>MAHHHHHHMTRAFNFSAGPATLPESVLRQAQAEMLDWHGSGASIVEMSHRGAEFMSVAAEAEADLRRLLDIPDDYAVLFLSGGATTQQALIPLNFAAPGQRADYVVSGHWGKTAVKQAGVYVDVNIAASSEANGYRELPARADWQLSRDAAYVHITANETIHGVEFRDVPDTGNVPLIADFSSSIASEPLDVRRYGVIYAGAQKNLGPVGVAVMIIRRDLLERSGQPRADIFDYRSHVARDSMLNTPPTWNWYLAGLVFKWMLAEGGVTEFAKRNAAKAALVYGAIDGSGGFYRNEVAYAARSRMNIPFFLPDAELD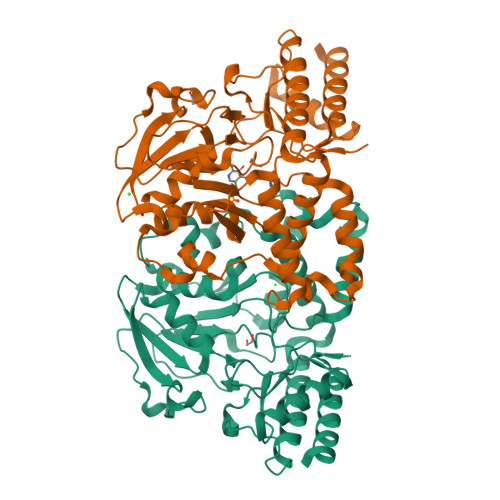ARFVAEAKAAGLLALKGHKVVGGIRASLYNAMPLAGAEALVAFMADFQQRHG[4x]>MGLELEWMPIEDLKLPSNVIEIIKKRGIKKLNPPQTEAVKKGLLEGNRLLLTSPTGSGKTLIAEMGIISFLLKNGGKAIYVTPLRALTNEKYLTFKDWELIGFKVAMTSGDYDTDDAWLKNYDIIITTYEKLDSLWRHRPEWLNEVNYFVLDELHYLNDPERGPVVESVTIRAKRRNLLALSATISNYKQIAKWLGAEPVATNWRPVPLIEGVIYPERKKKEYNVIFKDNTTKKVHGDDAIIAYTLDSLSKNGQVLVFRNSRKMAESTALKIANYMNFVSLDENALSEILKQLDDIEEGGSDEKELLKSLISKGVAYHHAGLSKALRDLIEEGFRQRKIKVIVATPTLAAGVNLPARTVIIGDIYRFNKKIAGYYDEIPIMEYKQMSGRAGRPGFDQIGESIVVVRDKEDVDRVFKKYVLSDVEPIESKLGSERAFYTFLLGILSAEGNLSEKQLENFAYESLLAKQLVDVYFDRAIRWLLEHSFIKEEGNTFALTNFGKRVADLYINPFTADIIRKGLEGHKASCELAYLHLLAFTPDGPLVSVGRNEEEELIELLEDLDCELLIEEP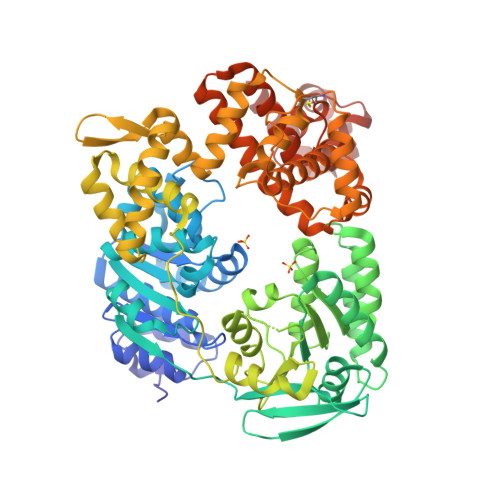YEEDEYSLYINALKVALIMKDWMDEVDEDTILSKYNIGSGDLRNMVETMDWLTYSAYHLSRELKLNEHADKLRILNLRVRDGIKEELLELVQISGVGRKRARLLYNNGIKELGDVVMNPDKVKNLLGQKLGEKVVQEAARLLNRFH[2x]> AFVVTDN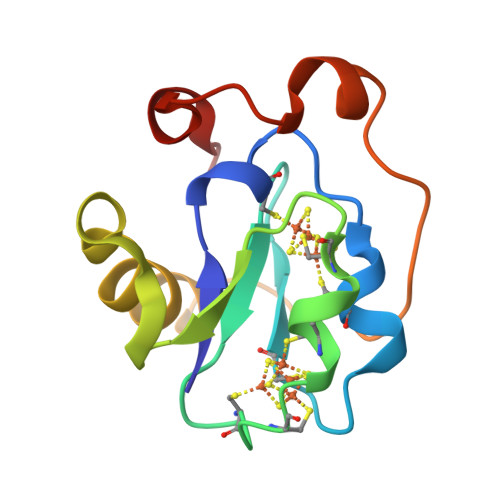CIKCKYTDCVEVAPVDCFYEGPNFLVIHPDECIDCALCEPECPAQAIFSEDEVPEDMQEFIQLNAELAEVWPNITEKKDPLPDAEDWDGVKGKLQHLER>XVDAAVAKVCGSEAIKANLRRSWGVLSADIEATGLMLMSNLFTLRPDTKTYFTRLGDVQKGKANSKLRGHAITLTYALNNFVDSLDDPSRLKCVVEKFAVNHINRKISGDAFGAIVEPMKETLKARMGNYYS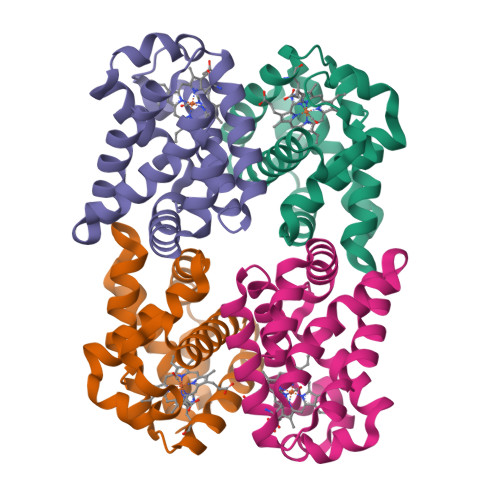DDVAGAWAALVGVVQAAL[4x];>XSRVAELANAVVSNADQKDLLRMSWGVLSVDMEGTGLMLMANLFKTSPSAKGKFARLGDVSAGKDNSKLRGHSITLMYALQNFVDALDDVERLKCVVEKFAVNHINRQISADEFGEIVGPLRQTLKARMGNYFDEDTVAAWASLVAVVQAAL[4x]> SARPSSSMADFRKFFAKAKHIVIISGAGVSAESGVPTFRGAGGYWRKWQAQDLATPLAFAHNPSRVWEFYHYRREVMGSKEPNAGHRAIAECETRLGK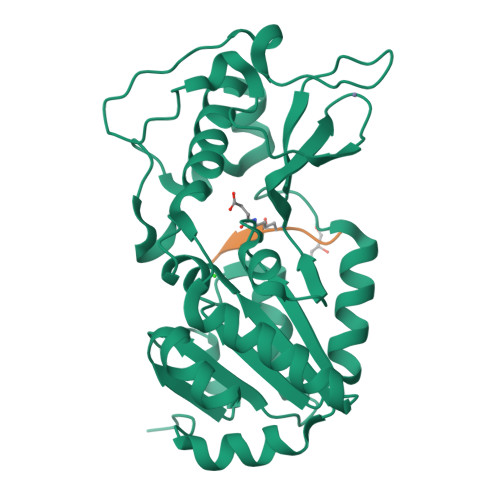QGRRVVVITQNIDELHRKAGTKNLLEIHGSLFKTRCTSCGVVAENYKSPICPALSGKGAPEPGTQDASIPVEKLPRCEEAGCGGLLRPHVVWFGENLDPAILEEVDRELAHCDLCLVVGTSSVVYPAAMFAPQVAARGVPVAEFNTETTPATNRFRFHFQGPCGTTLPEALA;> AVTXYTS>[2x]STSDGDDLFVPVSNFDPKSIFPEIKHPFEPMYANTENGKIVPTNSWISNLFYPSADNLAPTTPDPYTLRLLDGYGGNPGLTIRQPSAKVLGSYPPTNDVPYTDAGYMINSVVVDLRLTSSEWSDVVPDRQVTDWDHLSANLRLSTPQDSNSYIDFPIVRGMAYITANYNNLTPQFLSQHAIISVEADEKKSDDNTSTFSGRKFKITMNDDPTSTFIIYSLGDKPLELRKQDNSNLVASKPYTGVIRVAKLPAPEFETLLDASRAVWPTGGDISARSDDNNGASYTIKWKTNSNEAPLLTYAYAHHLTSIDDSNVKRTDMTLQSATKGPMTALVGNEWTLRETELSPVEWLPLQAAPNPTTINEIMTEINKDIASNYTQETAKEDNYFSGKGLQKFAMLALILNKSDQTQLRNPELAQIALDKLKAAFLPYLQNEQADPFRYDTLYKGIVAKAGLPTSMGGT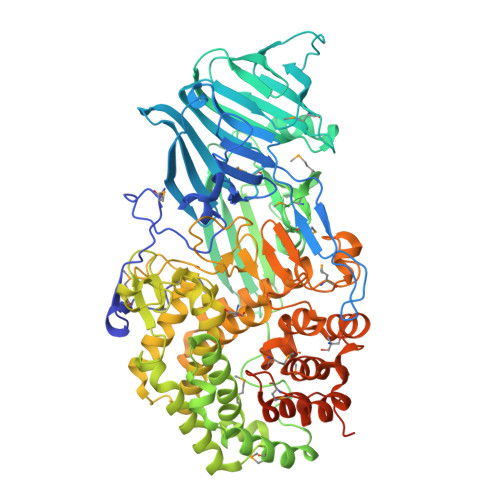DDLSAEFGHSYYSDHHYHQGYFVVTAAIIHHLDPTWNADRLKAWTEALIRDVNNANDGDEYFAAFRNWDWFAGHSWAGGIKPDGALDGRDQESVPESVNFYWGAKLWGLATGNTPLTKLASLQLAVTKRTTYEYFWMLDGNKNRPENIVRNKVIGIYFEQKTDYTTYFGRFLEYIHGIQQLPMTPELMEYIRTPEFVSQEWDEKLGAIAPTVQSPWAGVLYLNYAIINPAEAYPALRKVQMDDGQTRSYSLYLTATRPHFFRRSLLAALARHGSTRRPSLPSSGDDDKHEDGFLLRFRRLNPFNLKHRIY> MTLSILVAHDLQRVIGFENQLPWHLPNDLKHLKKLSTGHT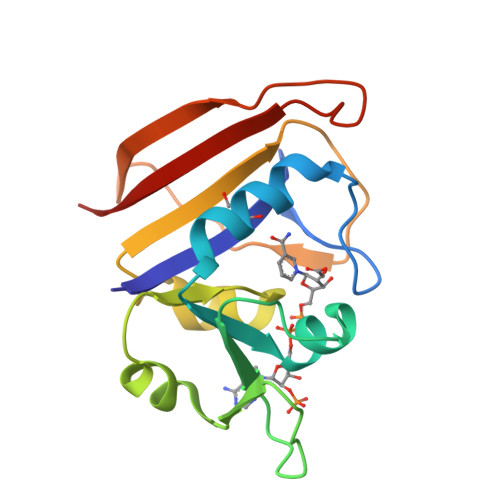LVMGRKTFESIGKPLPNRRNVVLTSDTSFNVEGVDVIHSIEDIYQLPGHVFIFGGQTLYEEMIDKVDDMYITVIEGKFRGDTFFPPYTFEDWEVASSVEGKLDEKNTIPHTFLHLIRKLE>MGESERSEAFGIPRDSPLSSGDAAELEQLRREAAVLREQLENAVGSHAPTRSARDIHQLEARIDSLAARNSKLMETLKEARQQLLALREEVDRLGQPPSGYGVLLATHDDDTVDVFTSGRKMRLTCSPNIDAASLKKGQTVRLNEALTVVEAGTFEAVGEISTLREILADGHRALVVGHADEERVVWLADPLIAEDLPDGLPEALNDDTRPRKLRPGDSLLVDTKAGYAFERIPKAEVEDLVLEEVPDVSYADIGGLSRQIEQIRDAVELPFLHKELYREYSLRPPKGVLLYGPPGCGKTLIAKAVANSLAKKMAEVRGDDAHEAKSYFLNIKGPELLNKFVGETERHIRLIFQRAREKASEGTPVIVFFDEMDSIFRTRGTGVSSDVETTVVPQLLSEIDGVEGLENVIVIGASNREDMIDPAILRPGRLDVKIKIERPDAEAAQDIYSKYLTEFLPVHADDLAEFDGDRSACIKAMIEKVVDRMYAEIDDNRFLEVTYANGDKEVMYFKDFNSGAMIQNVVDRAKKNAIKSVLETGQPGLRIQHLLDSIVDEFAENEDLPNTTNPDDWARISGKKGERIVYIRTLVTGKSSSASRAIDTESNLGQYL[6x];> GSMAQEQTKRGGGGGDDDDIAGSTAAGQERREKLTEETDDLLDEIDDVLEENAEDFVRAYVQKGGQ

Proteasomes are present in eukaryotes, archaea and Actinobacteria, including the human pathogen Mycobacterium tuberculosis, where proteasomal degradation supports persistence inside the host. In mycobacteria and other members of Actinobacteria, prokaryotic ubiquitin-like protein (Pup) serves as a degradation tag post-translationally conjugated to target proteins for their recruitment to the mycobacterial proteasome ATPase (Mpa). The bacterial 20S proteasome interacts with a ring-shaped AAA regulatory complex called the mycobacterial proteasome ATPase (Mpa) in mycobacteria or ARC (ATPase forming ring-shaped complexes) in other actinobacterial species. Here, we use single-particle cryo-electron microscopy to determine the structure of Mpa in complex with the 20S core particle at an early stage of pupylated substrate recruitment, shedding light on the mechanism of substrate translocation.

To improve the local resolution of Mpa, we performed local 3D classification and 3D refinement combined with signal subtraction of the 20S CP (see “Methods”). This approach resolved two states of Mpa at an average resolution of 3.8 Å and 3.9 Å, respectively. The two states correspond to two distinct motor conformations stalled at sequential stages of substrate translocation. Based on the visible side-chain density, this tubular EM-density can be assigned to the first 15 residues of the Mtb Pup sequence. A stacked pair of residues, the canonical aromatic pore loop residue F341 and the highly conserved adjacent lysine residue K340, forms a spiral-staircase that encircles the Pup N-terminal segment by engaging in unspecific interactions with its Cα backbone. Another channel loop about 16–17 Å further down (V384-S385-S386) forms a second spiral-staircase. It is resolved only in four of the six protomers, the other loops are flexible, as the Pup N-terminal segment has not yet reached far enough down at this state of engagement. In state A, 5 of the 6 protomers of Mpa are in the ATP-bound state with arginine fingers contributed by the neighboring subunit. The protomer with the pore loop at the bottom of the staircase (protomer 6, cyan) displays weak nucleotide density corresponding to the ADP nucleotide form. In this case, the arginine finger from the neighboring subunit is displaced and moved away from the bound nucleotide.> QDYGGTAALLTS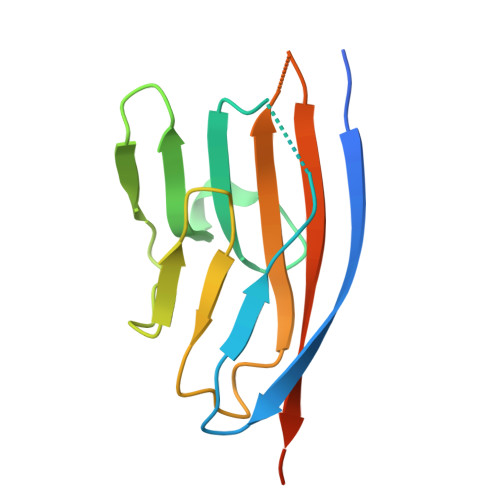KEMRFSAAEGAKVLLSVPDQEENLLSFSWYKGKDVNENFTIAHYKKSSDSLQLGKKVSGREEIYKDGSMMLRAITLEDTGFYTLQTFKAHGQQEVTHVHLQVYKIVTKAENLYF> MGSDKIHHHHHHMNAPLSHSRPMMQPSEDKSLATVFPFAGRVLDETPMLLGEGPTFDPASGTAWWFNILERELHELHLASGRKTVHALPFMGSALAKIS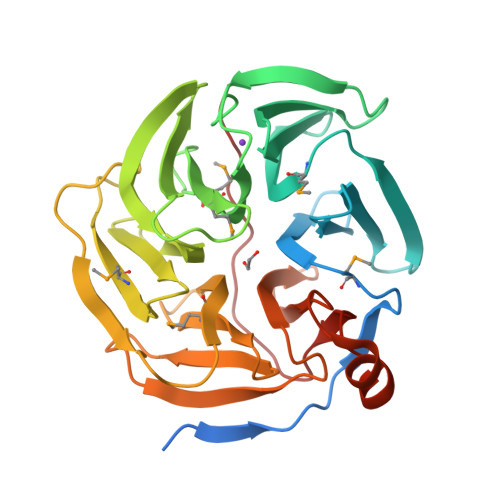DSKQLIASDDGLFLRDTATGVLTLHAELESDLPGNRSNDGRMHPSGALWIGTMGRKAETGAGSIYHVAKGKVTKLFADISIPNSICFSPDGTTGYFVDTKVNRLMRVPLDARTGLPTGKAEVFIDSTGIKGGMDGSVCDAEGHIWNARWGEGAVDRYDTDGNHIARYEVPGKQTTCPAFIGPDASRLLVTSAREHLDDDAITANPQHGLTFELGIEVKGRFEPLYRL>MALSVHPSIGVARLGNANTDNFVLNPMEIGGLPYEHDVDLKPTTTVVNFKDEAGCIRRQGQVFKVFGASNEELTLDSPNVKNIEWTVHLANKKAAWYEFRELNGNLLYGRDNSYSARGVPWRNASKTASSERQSLIIDLGPRSVSGVMATVEISINNIPETYLHPSYPSGELLQGSKHFESLGTLRTDSQGRLIVLGGYGFAGGNTDLSGYGGGDDWYDDISDGSVTCVVTYSDDSSETSTAWMVVGSPDFAPEIVNISTLSDTCFDVGVRNFDLVPDMYDSATGHYKSDYVANFDRDILPIIQRISQYQWVSNVQSMSGFFSFQFDYRDGSAANKANRMKYYNYFRQLDNKVIGDYDQPQQVLMSSEVEGDILPLMPMNSGSNSVSSSNFYDLTDNVVEKFLALDATQLFLLGQWAEGEFTAGPADDYPVSDMDTASIGNCVGLPMCPGIEMTWSLQNPVIYKDAYQIKHYQDKAYFDVNGLTPERDECEEETGCEPGDLTKRMACPWQADFFNCTIQTVNFSEPS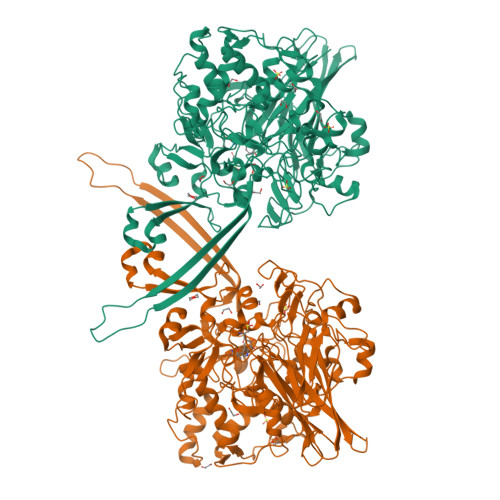VNKASQTETVTSRTHYEWGNLPAGVSVPDQSSVSATKNVDEKVPLPPAYYSYWWPPQSPWDVLTGELDTEGQLHSHLPAGQQINYARGINSYSQMVEHWSALAFIRDRNQNNDGFPFFTETERNHELFDFKEVLVGQVTGNSEDNETSLPVFFINANKESLEGKGTKKGKLMASYFEERAFSKVRSSNIRPRSGTRMRG[2x]> ADLANGAKVFSGNCAACHMGGGNVV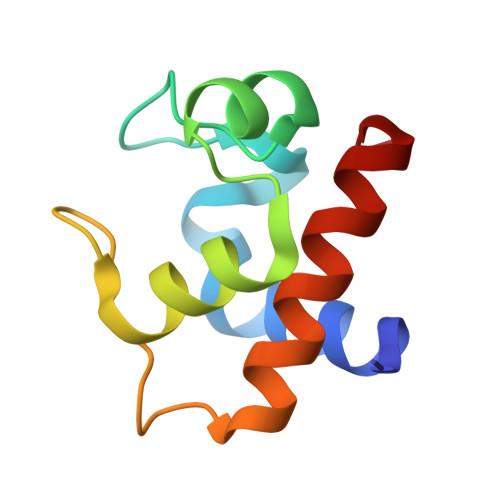MANKTLKKEALEQFGMYSEDAIIYQVQHGKNAMPAFAGRLTDEQIQDVAAYVLDQAAKGWV>[2x]PDISQSYWTVWGMRKNEALVRFLEAEDFDAAIIFVRTKNATLEVAEALERNGYNSAALNGDMNQALREQTLERLKDGRLDILIATDVAARGLDVERISLVVNYDIPMDSESYVHRIGR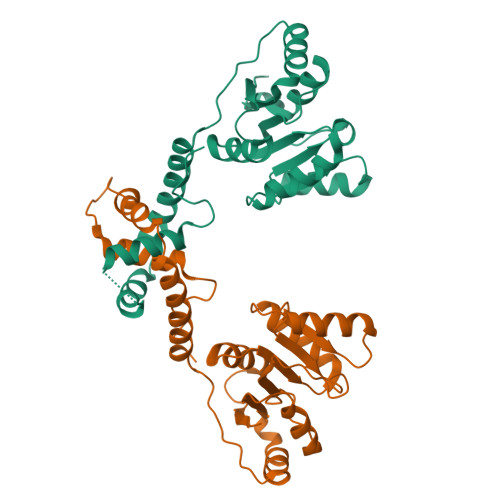TGRAGRAGRALLFVENRERRLLRNIERTMKLTIPEVELPNAELLGKRRLEKFAAKVQQQLESSDLDQYRALLSKIQPTAEGEELDLETLAAALLKMAQGERTLIVPPDAP ethyl (3S)-3-hydroxy-4-({(2S)-4-methyl-1-[(3-methylbutyl)amino]-1-oxopentan-2-yl}amino)-4-oxobutanoate 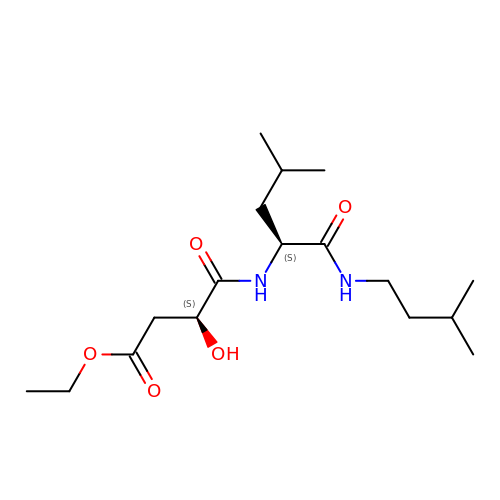| C17 H32 N2 O5 | FGRTVYZNNRCSAS-KBPBESRZSA-N>[2x]MDIWYGTAAVPKDLDNSAVTIGVFDGVHRGHQKLINATVEKAREVGAKAIMVTFDPHPVSVFLPREAPLGITTLAERFALAESFGIDGVLVIDFTRELSGTSPEKYVEFLLEDTLHASHVVVGANFTFGENAAGTADSLRQICQSRLTVDVIDLLDDEGVRISSTTVREFLSEGDVARANWALGRHFYVTGPVVR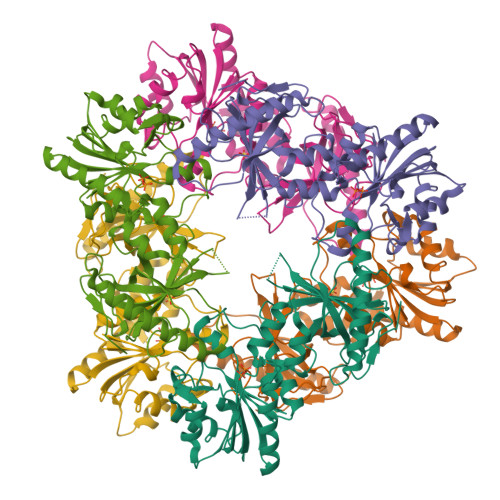GAGRGGKELGFPTANQYFHDTVALPADGVYAGWLTILPTEAPVSGNMEPEVAYAAAISVGTNPTFGDEQRSVESFVLDRDADLYGHDVKVEFVDHVRAMEKFDSVEQLLEVMAKDVQKTRTLLAQDVQAHKMAPETYFLQAES>[60x]AKLETVTLGNIGKDGKQTLVLNPRGVNPTNGVASLSQAGAVPALEKRVTVSVSQPSRNR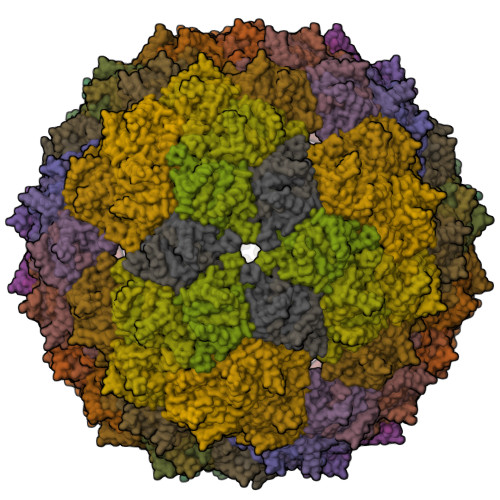KNYKVQVKIQNPTACTANGSCDPSVTRQAYADVTFSFTQYSTDEERAFVRTELAALLASPLLIDAIDQLNPAY To design a specific inhibitor of colibactin biosynthesis, we targeted the colibactin-activating enzyme ClbP. This membrane-embedded periplasmic serine peptidase is essential for the genotoxicity of pks+ E. coli.

To address this need, we designed and characterized a series of boronic acid-based inhibitors of colibactin biosynthesis. Using biochemical assays and crystallography, we show that they engage the ClbP binding pocket, forming a covalent bond with the catalytic serine. In this structure, the d-Asn side chain of the inhibitor projects into a tight-fitting pocket and hydrogen bonds with the side chains of residues S188, H257 and N331. N331 also hydrogen bonds to E92, setting its orientation and helping to enforce ClbP’s selectivity for d-Asn- over d-Asp-containing substrates. The inhibitor-bound structure of ClbP also reveals continuous electron density from the S95 side chain to the ligand, indicating essentially complete conversion to a covalent protein–inhibitor complex. This boronate complex is a structural analog of the tetrahedral intermediates formed during amide bond hydrolysis and participates in several stabilizing interactions that are likely relevant to the activation of precolibactin. The backbone amides of Q330 and S95 hydrogen bond to one of the boronate oxygen atoms and are thus well positioned to stabilize the negative charge that accumulates upon formation of the covalent bond with S95. In addition, Y186, which is part of the catalytic triad that defines this enzyme family, is positioned to stabilize this complex by donating a hydrogen bond to either the other boronate oxygen atom or the oxygen nucleophile on the serine side chain. Thus, the potency of these ClbP inhibitors arises both from their ability to mimic the hydrogen-bonding interactions of intermediates in the hydrolysis of precolibactin and the formation of a covalent bond with the catalytic serine residue.

> QEHEPIGAQDERLSTLIHQRMQEAKVPALSVSVTIKGVRQRFVYGVADVASQKANTLDTVYELGSMSKAFTGLVVQILIQEGRLRQGDDIITYLPEMRLNYQGKPASLTVADFLYHTSGLPFSTLARLENPMPGSAVAQQLRNENLLFAPGAKFSYASANYDVLGAVIENVTGKTFTEVIAERLTQPLGMSATVAVKGDEIIVNKASGYKLGFGKPVLFHAPLARNHVPAAYIHSTLPDMEIWIDAWLHRKALPATLREAMSNSWRGNSDVPLAADNRILYASGWFIDQNQGPYISHGGQNPNFSSCIALRPDQQIGIVALANMNSNLILQLCADIDNYLRIGKYADGAGDAITATDTLFVYLTLLLCFWGAVVVVRGAFRVYRATAHGPGKQQRLRLRVRDYIIALAVPGLVAAMLYVAPGILSPGLDWRFILVWGPSSVLAIPFGIILLAFVLTLNHQIKRILLHNKEWDDEHHHHHH> GLEDDLVEVIVDKAQQTLASIKSDSKHTQKVPSLTANETGATLPTTPSDSVETRTTLMHYTGSETTLENF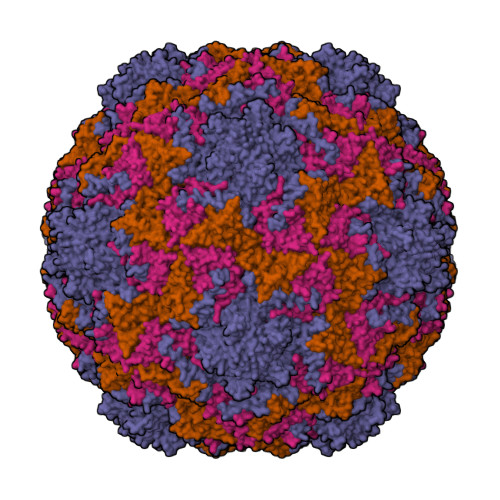LGRAACVHVVEIVNKRPTDTEEHRMQLLFNNWKINLSSLVQLRRKLEMFTYVRFDSEYTIIATSSQPNEAKFSSNLTIQAMFIPPGAPNPKKWDDYTWQSATNPSVFFNVGKSARFSVPYLGIASAYNCFYDGYSHDNSTTPYGINVLNHMGSMAFRVVNEHDNHTTHVKVRVYHRAKHIRAWVPRAPRALEYLHIGRTNYKQSPQNPIKTRKTISTY;> GYSDRVEQITLGNSTITTQEAANSIVAYGEWPSFLSDVDASDVNKTTKPDTSACRFYTLDSKMWTQGSKGWCWKLPDALKDMGIFGQNMFFHSQGRTGYTIHVQCNATKFHSGCLLVVVIPEHQLASAEGGNVSVLYDKTHPGEKGIDLSEADSTGPMKDPLYMMDGTLIGNSLIFPHQFINLRTNNTATIVVPYINSVPMDSMTRHNNLSLMVIPIVDITATSGTTPSIPVTITIAPMFLELSGIRSKAVI;> GLPTVLTPGSEQFLTTDDRQSPSAMPNYEPTPLIHIPGEVKNLLEIAQVDTLIPLNNTTNTTGLGMYRIPLVQNMQGEQVFGFRLYLGDGVLKTTLLGELCQYFTHWAGSLRLSFMYTGPALSSAKLLIAYTPPGAQGPTKRKEAMLGTHVVWDIGLQSTVVLNIPWTSGVQYRYTDPDTYTSAGFVSCWYQTSLVLPPQTQQTVYMLGFISACPDFKLRLMKDTQSIHQ;> MGAQVSTQKSGSHENQNILTNGSNQTFTVINYYKDAASSSSAGQSFSMDPSKFTEPVKDIMLKGAPALN(1S,2S)-cyclohexane-1,2-diol | C6 H12 O2 | 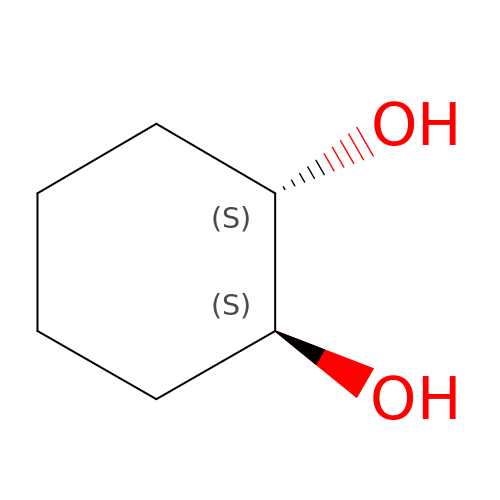PFURGBBHAOXLIO-WDSKDSINSA-N N-{3-[(2R)-6-amino-2,4-dimethyl-3-oxo-2,3,4,5-tetrahydropyrazin-2-yl]phenyl}-5-chloropyridine-2-carboxamide 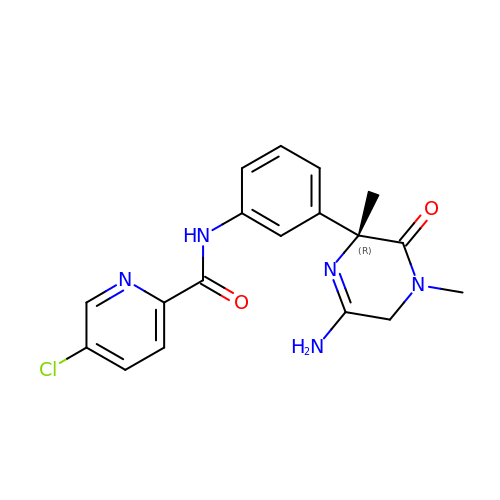| C18 H18 Cl N5 O2 | MRYFMHAPTQCQLE-GOSISDBHSA-N>MTQETTTLTGQSPPPVRDWPALDLDGPEFDPVLAELMREGPLTRVRLPHGEGWAWLATRYDDVKAITNDPRFGRAEVTQRQITRLAPHFKPRPGSLAFADQPDHNRLRRAVAGAFTVGATKRLRPRAQEILDGLVDGILAEGPPADLVERVLEPFPIAVVSEVMGVPAADRERVHSWTRQIISTSGGAEAAERAKRGLYGWITETVRARAGSEGGDVYSMLGAAVGRGEVGETEAVGLAGPLQIGGEAVTHNVGQMLYLLLTRRELMARMRERPGARGTAL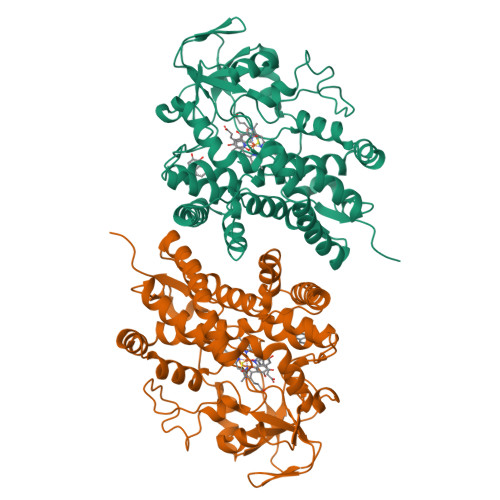DELLRWISHRTSVGLARIALEDVEVHGTRIAAGEPVYVSYLAANRDPDVFPDPDRIDLDRDPNPHLAYGNGHHFCTGAVLARMQTELLVDTLLERLPGLRLAVPAEQVAWRRKTMIRGPRTLPCTWHHHHHH[2x]6-{[(3R,4R)-4-{2-[(2,2-difluoro-2-phenylethyl)amino]ethoxy}pyrrolidin-3-yl]methyl}-4-methylpyridin-2-amine | C21 H28 F2 N4 O 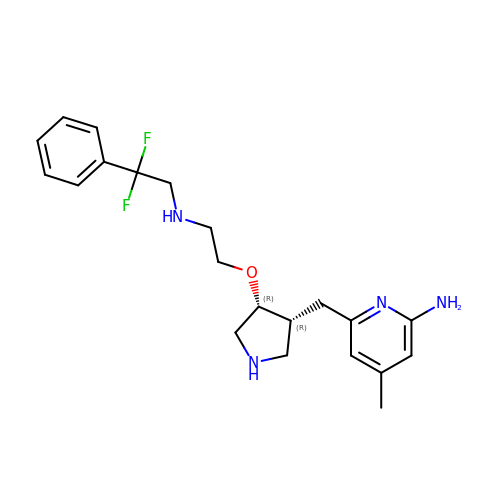| RTMROEXMNLIGEG-APWZRJJASA-N> WLYSTNAKDIAVLYFMLAIFSGMAGTAMSLIIRLELAAPGSQYLHGNSQLFNVLVVGHAVLMIFFLVMPALIGGFGNYLLPLMIGATDTAFPRINNIAFWVLPMGLVCLVTSTLVESGAGTGWTVYPPLSSIQAHSGPSVDLAIFALHLTSISSLLGAINFIVTTLNMRTNGMTMHKLPLFVWSIFITAFLLLLSLPVLSAGITMLLLDRNFNTSFFEVSGGGDPILYEHLF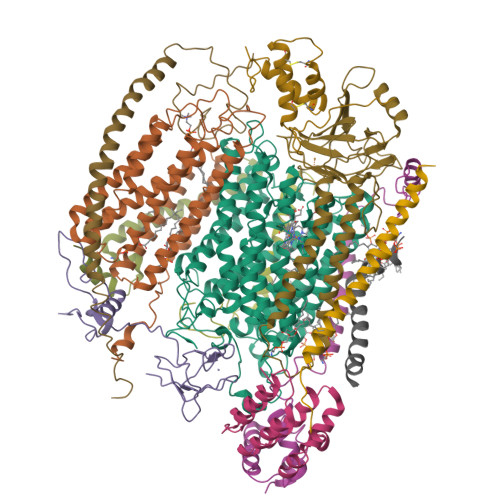WFFGHPEVYILIIPGFGIISHVVSTYSKKPVFGEISMVYAMASIGLLGFLVWSHHMYIVGLDADTRAYFTSATMIIAIPTGIKIFSWLATIHGGSIRLATPMLYAIAFLFLFTMGGLTGVALANASLDVAFHDTYYVVGHFHYVLSMGAIFSLFAGYYYWSPQILGLNYNEKLAQIQFWLIFIGANVIFFPMHFLGINGMPRRIPDYPDAFAGWNYVASIGSFIATLSLFLFIYILYDQLVNGLNNKVNNKSVIYNKAPDFVESNTIFNLNTVKSSSIEFLLTSPPAVHSFNTPAVQS;> DVPTPYACYFQDSATPNQEGILELHDNIMFYLLVILGLVSWMLYTIVMTYSKNPIAYKYIKHGQTIEVIWTIFPAVILLIIAFPSFILLYLCDEVISPAMTIKAIGYQWYWKYEYSDFINDSGETVEFESYVIPDELLEEGQLRLLDTDTSMVVPVDTHIRFVVTAADVIHDFAIPSLGIKVDATPGRLNQVSALIQREGVFYGACSELCGTGHANMPIKIEAVSLPKFLEWLNEQ;> THLERSRHQQHPFHMVMPSPWPIVVSFALLSLALSTALTMHGYIGNMNMVYLALFVLLTSSILWFRDIVAEATYLGDHTMAVRKGINLGFLMFVLSEVLIFAGLFWAYFHSAMSPDVTLGACWPPVGIEAVQPTELPLLNTIILLSSGATVTYSHHALIAGNRNKALSGLLITFWLIVIFVTCQYIEYTNAAFTISDGVYGSVFYAGTGLHFLHMVMLAAMLGVNYWRMRNYHLTAGHHVGYETTIIYTHVLDVIWLFLYVVFYWWGV;> VVKTAQNLAEVNGPETLIGPGAKEGTVPTDLDQETGLARLELLGKLEGIDVFDTKPLDSSRKGTMKDPIIIESYDDYRYVGCTGSPAGSHTIMWLKPTVNEVARCWECGSVYKLNPV;> ALSNAAVMDLQSRWENMPSTEQQDIVSKLSERQKLPWAQLTEPEKQAVWYISYGEWGPRRPVLNKGDSSFIAKGVAAGLLFSVGLFAVVRMAGGQDAKTMNKEWQLKSDEYLKSKNANPWGGYSQVQS;> ETFEEFTARYEKEFDEAYDLFEVQRVLNNCFSYDLVPAPAVIEKALRAARRVNDLPTAIRVFEALKYKVENEDQYKAYLDELKDVRQELGVPLKEELFP;> NKVIQLQKIFQSSTKPLWWRHPRSALYLYPFYAIFAVAVVTPLLYIPNAIRGIKA;> VHFKDGVYENIPFKVKGRKTPYALSHFGFFAIGFAVPFVACYVQLKKSGAF;> TIAPITGTIKRRVIMDIVLGFSLGGVMASYWWWGFHMDKINKREKFYAELAE;> NSPLHTVGFDARFPQQNQTKHCWQSYVDYHKCVNMKGEDFAPCKVFWKTYNALCPLDWIEKWDDQREKGIFAGDINSD;> NALKPAFGPPDKVAAQKFKESLMATEKHAKDTSNMWVKISVWVALPAIALTAVNTYFVEKEHAEHREHLKHVPDSEWPRDYEFMNIRSKPFFWGDGDKTLFWNPVVNRHIEHDD;> ESWVITEGRRLIPEIFQWSAVLSVCLGWPGAVYFFSKA(2S)-2-benzamido-4-methyl-pentanoic acid | C13 H17 N O3 | 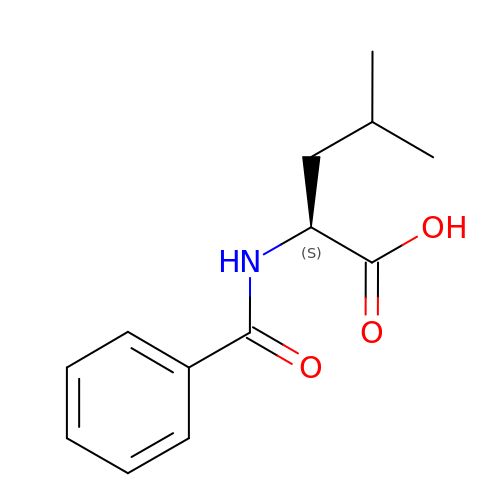POLGZPYHEPOBFG-NSHDSACASA-N>GANLHLLRQKIEEQAAKYKHSVPKKCCYDGARVNFYETCEERVARVTIGPLCIRAFNEC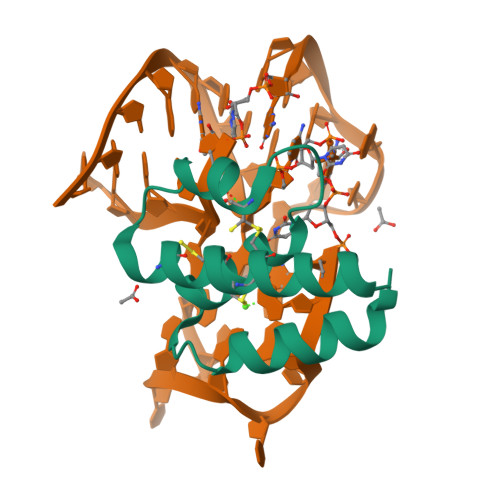CTIANKIRKESPHKPVQLGR[3x]>M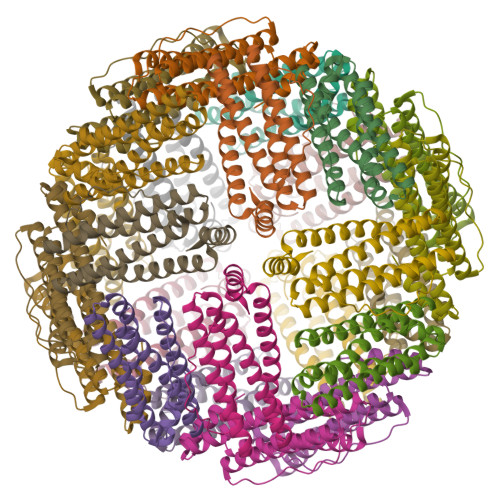LKPEMIEKLNEQMNLELYSSLLYQQMSAWCSYHTFEGAAAFLRRHAQEEMTHMQRLFDYLTDTGNLPRINTVESPFAEYSSLDELFQETYKHEQLITQKINELAHAAMTNQDYPTFNFLQWYVSEQHEEEKLFKSIIDKLSLAGKSGEGLYFIDKELSTLDTQN[6x]>AIPQKIRIGTDPTYAPFESKNAQGELVGFDIDLAKELCKRINTQCTFVENPLDALIPSLKAKKIDAIMSSLSITEKRQQEIAFTDKLYAADSRLVVAKNSDIQPTVASLKGKRVGVLQGTTQETFGNEHWAPKGIEIVSYQGQDNIYSDLTAGRIDAAFQDEVAASEGFLKQPVGKDYKFGGPAVKDEKLFGVGTGMGLRKEDNELREALNKAFAEMRADGTYEKLA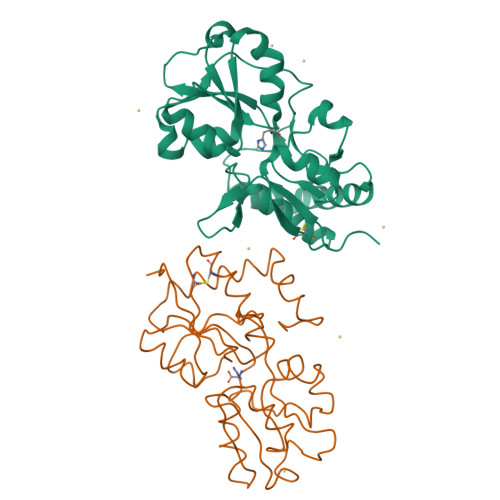KKYFDFDVYGG[2x]>METDTLLLWVLLLWVPGSTGDAAQPAARDQNAGFVKSPMSETKLTGDAFELYCDVVGSPTPEIQWWYAEVNRAESFRQLWDGARKRRVTVNTAYGSNGVSVLRITRLTLEDSGTYECRASNDPKRNDLRQNPSITWIRAQATISVLQKEDLYFQSHHHHHH[4x]

Plasma membrane Ca2+-ATPases (PMCAs) have a crucial role in this process by extruding Ca2+ against a steep concentration gradient from the cytosol to the extracellular space. Native PMCAs form heterodimeric assemblies with the small transmembrane proteins neuroplastin (NPTN) and basigin (BASI). Here we present the structures of mouse PMCA2 in the presence and absence of its accessory subunit neuroplastin in eight different stages of its transport cycle. The structures revealed an overall classical P-type ATPase architecture with ten transmembrane helices characteristic of the P2 subgroup.

NPTN was clearly resolved in all NPTN–PMCA2 structures, including the immunoglobulin-like domains Ig2 and Ig3. The most N-terminal Ig1 domain, however, was highly flexible and consequently less resolved. We therefore determined its structure by X-ray crystallography and fitted the resulting 2 Å structure into the density of the E1-Ca state. The resulting combined atomic model of NPTN represents, to our knowledge, the first complete structure of NPTN. The Ig2 and Ig1 domains of NPTN do not interact directly with PMCA2, but Ig2 appears rigidly tethered to Ig3 by means of two hydrogen bonds.> MASAATGVRAVPGNENSLEIEELARFAVDEHNKKENALLEFVRVVKAKEQIDLTQEWVFTMYYLTLEAKDGGKKKLYEAKVWVKG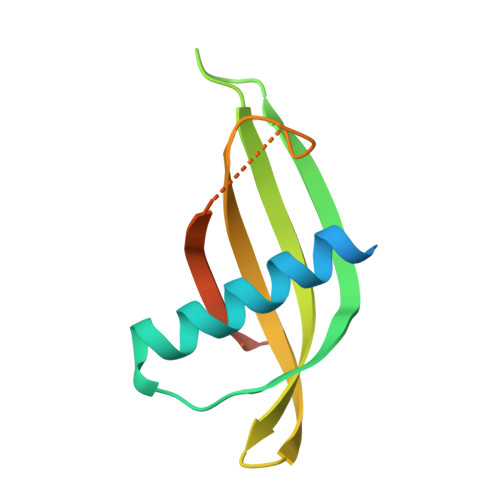LTNWKLGMNFKELQEFKPVGDAAAAHHHHHH> NGAAKIITIVPLVNDLDPLDILYKLLKCADDEGIMVQEVDSKRIFNVHIKKFKSNLKIIIPDMTNFLNILDCAKVADFVVFGLSGVQ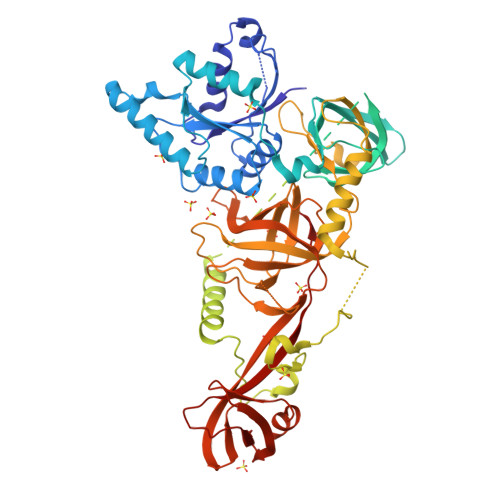EVDEEFGEQIIRALELQGIASYIGVISNLSAVHEKEKFQLDVKQSLESYFKHFFPSEERVYNLEKNSDALNVLRTLCQRLPRSINWRDNRGYVVADFVDFVETSPDSGDLVIEGTVRGIGFNANRLVHIPDFGDFQLNKIEKISESSQKRKIIKEKATDSLSLELDLQTVFESNMNRDTLDEYAPEGTEDWSDYDEDFEYDGLTTARYDDHGFLPGREQTSKKAAVPKGTSDYQAKWYLDDVIDANEEEEAEQTNGKDETMMEIDDEMMVEQDNEEVAGDEEYDIEDNEGFEELSPEEEERQLREFRDMEKEDREFPDEIELEPSESAIERLKRYRGLKNLYNCDWQVDEKDPSSPAEWKRLLRIGNYKNTKNRIIKETKNEAQAIAGDRIRMFIRFPKFLLEKIQDPKQLLFAVYGLLLHEHKNAVVNFSLQRWEQYDKPVPSQEPIVVQYGVRRYTIQPLFSQGSNSPNNVHKYERFLHPDTVSVATCIAPVDFTQSPAIFFKPSPTDAKNIELIGHGTFLNADHSRILAKRAILTGHPFRFHKTVVTVRYMFFRPEDVEWFKSIPLFTKSGRSGFIKESLGTHGYFKATFDGKLSAQDVVAMSLYKRMWPMPSLPWNGM> RDWVVAPISVPENGKGPFPQRLNQLKSNKDRDTKIFYSITGPGADSPPEGVFAVEKETGWLLLNKPLDREEIAKYELFGHAVSENGASVEDPMNISIIVTDQNDHKPKFTQDTFRGSVLEGVLPGTSVMQVTATDEDDAIYTYNGVVAYSIHSQEPKDPHDLMFTIHRSTGTISV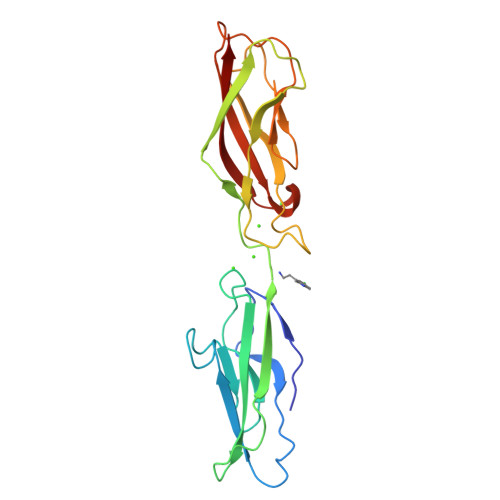ISSGLDREKVPEYTLTIQATDMDGDGSTTTAVAVVEILD> SQCSSTLVKHIKAPLHLVWSIV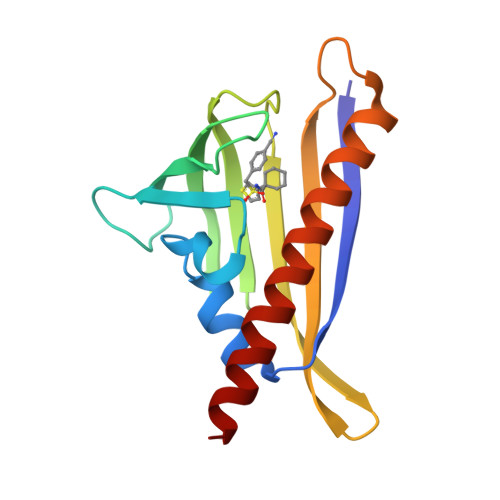RRFDEPQKYKPFISRCVVQGKKLEVGSVREVDLKSGLPATKSTEVLEILDDNEHILGIRIVGGDHRLKNYSSTISLHSETIDGKTGTLAIESFVVDVPEGNTKEETCFFVEALIQCNLNSLADVTERLQAESME>[2x]KKIFKPEELRQALMPTLEALYRQDPESLPFRQPVDPQLLGIPDYFDIVKNPMDLSTIKRKLDTGQYQEPWQYVDDVWLMFNNAWLYNRKTSRVYKFCSKLAEVFEQEIDPVMQSLG

Many proteins, including the EP300/CBP histone acetyltransferases (HATs), contain several targetable domains. EP300 and CBP broadly regulate the activity of other proteins through their protein acetyltransferase catalytic activity. These proteins contain several highly homologous domains, including KIX, bromodomains (BRDs) and HAT domains, through which they interact with, dock to, and acetylate target proteins, respectively. EP300/CBP are critical gene-regulatory targets in cancer, with existing high potency inhibitors of either the catalytic HAT domain or protein-binding bromodomain (BRD). Using crystallography, we identify the binding mechanism of the EP300/CBP-specific BRD inhibitor CCS1477 in complex with the EP300, CBP and BRD4 BRDs, and define components of the CCS1477 catalytic binding core that are required for compound activity.

Since recombinant CBP BRD was more robust in biochemical assays and crystallization studies, Kd values were determined for all compound-CBP interactions by MST, and co-crystal structures of the CBP BRD with five of the seven analogues were determined. Introducing bis-trifluoromethyl in meta position of the phenyl ring (compound 4) reduced the binding affinity by ~40-fold; while the co-crystal structure revealed Pi-cation and hydrogen-bonding interactions with R1173, steric hindrance imposed on the LPF shelf leads to conformational changes that negatively impact overall binding affinity. While none of the analogues were superior to CCS1477 in terms of binding affinity, substitutions were well tolerated if productive interactions with R1173 were maintained.>MSAIENFDAHTPMMQQYLRLKAQHPEILLFYRMGDFYALFYDDAKRASQLLDISLTKRGASAGEPIPMAGIPYHAVENYLAKLVNQGESVAICEQIGDPATSKGPVERKVVRIVTPGTISDEALLQERQDNLLAAIWQDSKGFGYATLDISSGRFRLSEPADRETMAAELQRTNPAELLYAEDFAEMSLIEGRRGLRRRPLWEFEIDTARQQLNLQFGTRDLVGFGVENAPRGLCAAGCLLQYAKDTQRTTLPHIRSITMEREQDSIIMDAATRRNLEITQNLAGGAENTLASVLDCTVTPMGSRMLKRWLHMPVRDTRVLLERQQTIGALQDFTAGLQPVLRQVGDLERILARLALRTARPRDLARMRHAFQQLPELRAQLETVDSAPVQALREKMGEFAELRDLLERAIIDTPPVLVRDGGVIASGYNEELDEWRALADGATDYLERLEVRERERTGLDTLKVGFNAVHGYYIQISRGQSHLAPINYMRRQTLKNAERYIIPELKEYEDKVLTSKGKALALEKQLYEELFDLLLPHLEALQQSASALAELDVLVNLAERAYTLNYTCPTFIDKPGIRITEGRHPVVEQVLNEPFIANPLNLSPQRRMLIITGPNMGGKSTYMRQTALIALMAYIGSYVPAQKVEIGPIDRI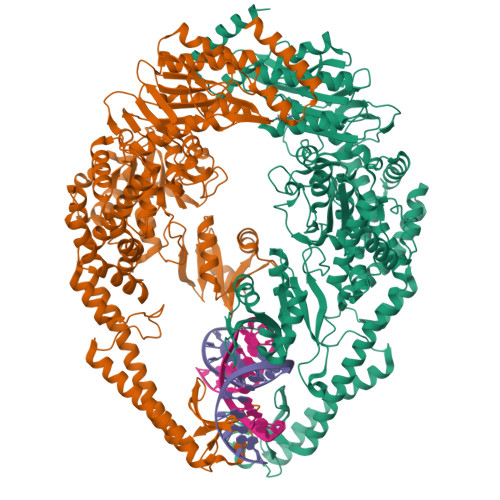FTRVGAADDLASGRSTFMVEMTETANILHNATEYSLVLMDEIGRGTSTYDGLSLAWACAENLANKIKALTLFATHYFELTQLPEKMEGVANVHLDALEHGDTIAFMHSVQDGAASKSYGLAVAALAGVPKEVIKRARQKLRELESIS[2x]> SGRSRLLEDFRNQRYPNLQLRDLANHIVEFSQDQHGSRFIQQKLERATAAEKQMVFSEILAAAYSLMTDVFGNYVIQKFFEFGTPEQKNTLGMQVKGHVLQLALQMYGCRVIQKALESISPEQQQEIVHELDGHVLKCVKDQNGNHVVQKCIECVDPVALQFIINAFKGQVYSLSTHPYGCRVIQRILEHCTAEQTTPILDELHEHTEQLIQDQYGNYVIQHVLEHGKQEDKSILINSVRGKVLVLSQHKFASNVVEKCVTHATRGERTGLIDEVCTFNDNALHVMMKDQYANYVVQKMIDVSEPTQLKKLMTKIRPHMAALRKYTYG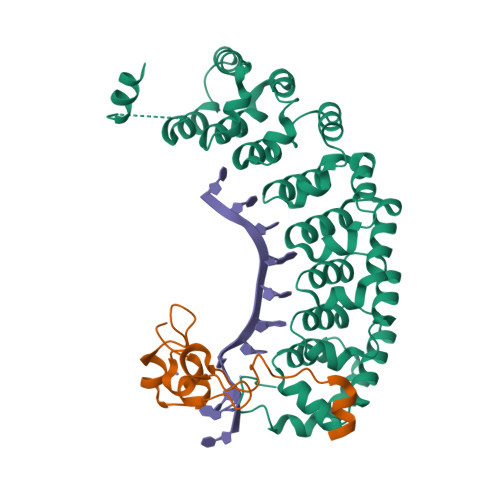KHINAKLEK;> SRGASNSSNNNNNNNKVYKRYNSKAKEISRHCVFCENNNEPEAVINSHSVRDNFNRVLCPKLRTYVCPICGASGDSAHTIKYCPKKPIITMEDAIKAESFRLAKSSYYKQQMKVV> YSDPKEYIESKYYDALFSIHTPLAYFV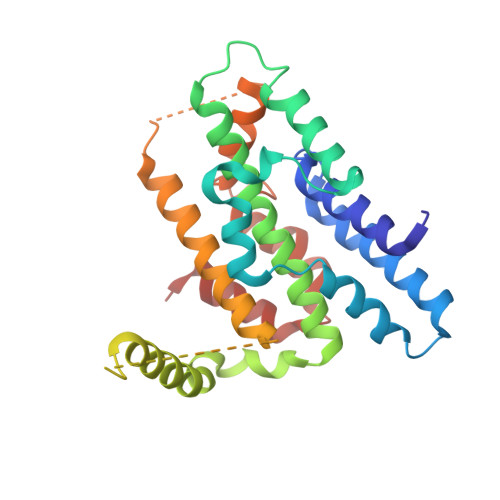KSNLVRLKNTCRTKYGSDSYKIAYQAMLQKFLLSIVQFKDRHDNRLLLEPFSSPIADEKRKNCLTKFVIQDENKNSSTIADLCVVLKSREIKLQILLLLEIIGLNDLDWNFRDFEKKYKLKLKKRSLNLTKKGLVRRRSKKKTSEKDKGIERITTSLDYCEQLDLYLDRACILDILLSSETPNPDAIEASNGTIQEHKKNILDKSKEASLVGFINYVLIPYFNKKVPHAVEFIIQKLKGP> ETGSKSSWGLENEALIVRCPQRGRSTYPVEWYYSDTNESIPTQKRNRIFVSRDRLKFLPARVEDSGIYACVIRSPNLNKTGYLNVTIHKKPPSCNIPDYLMYSTVRGSDKNFKITCPTIDLYNWTAPVQWFKNCKALQEPRFRAHRSYLFIDNVTHDDEGDYTCQFTHAENGTNYIVTATRSFTVEEKGFSMFPVITNPPYNHTMEVEIGKPASIACSACFGKGSHFLADVLWQINKTVVG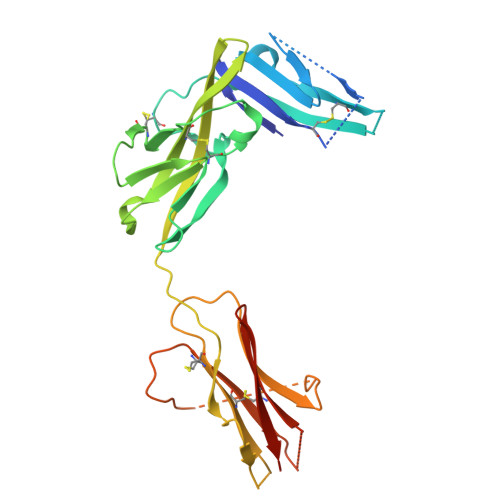NFGEARIQEEEGRNESSSNDMDCLTSVLRITGVTEKDLSLEYDCLALNLHGMIRHTIRLRRKHHHHHH> DLDCGIPESIENGKVEDPESTLFGSVIRYTCEEPYYYMENGGGGEYHC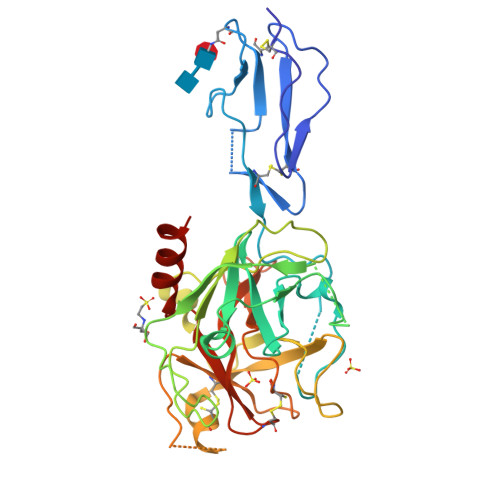AGNGSWVNEVLGPELPKCVPVCGVPREPFEEKQRIIGGSDADIKNFPWQVFFDNPWAGGALINEYWVLTAAHVVEGNREPTMYVGSTSVQTSRLAKSKMLTPEHVFIHPGWKLLAVPEGRTNFDNDIALVRLKDPVKMGPTVSPICLPGTSSDYNLMDGDLGLISGWGRTEKRDRAVRLKAARLPVAPLRKCKEVKVEKPTADAEAYVFTPNMICAGGEKGMDSCKGDSGGAFAVQDPNDKTKFYAAGLVSWGPQCGTYGLYTRVKNYVDWIMKTMQENSTPRED> MVPISPIETVPVKLKPGMDGPKVKQWPLTEEKIKALVEICTEMEKEGKISKIGPENPYNTPVFACKKKDSTKWRKLVDFRELNKRTQDFWEVQLGIPHPAGLKKKKSVTVLDVGDAYFSVPLDEDFRKYTAFTIPSINNETPGIRYQYNVLPQGWKGSPAIFQSSMTKILEPFKKQNPDIVIYQYIDDLYVGSDLEIGQHRTKIEELRQHLLRWGLTTPDKKHQKEPPFLWMGYELHPDKWTVQPIVLPEKDSWTVNDIQKLVGKLNWASQIYPGIKVRQL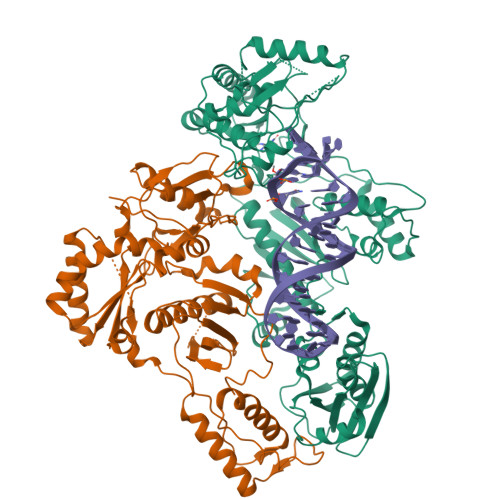SKLLRGTKALTEVIPLTEEAELELAENREILKEPVHGVYYDPSKDLIAEIQKQGQGQWTYQIYQEPFKNLKTGKYARMRGAHTNDVKQLTEAVQKITTESIVIWGKTPKFKLPIQKETWETWWTEYWQATWIPEWEFVNTPPLVKLWYQLEKEPIVGAETFYVDGAANRETKLGKAGYVTNKGRQKVVPLTNTTNQKTELQAIYLALQDSGLEVNIVTNSQYALGIIQAQPDKSESELVNQIIEQLIKKEKVYLAWVPAHKGIGGNEQVDKLVSA;> PISPIETVPVKLKPGMDGPKVKQWPLTEEKIKALVEICTEMEKEGKISKIGPENPYNTPVFAIKKKDSTKWRKLVDFRELNKRTQDFWEVQLGIPHPAGLKKKKSVTVLDVGDAYFSVPLDEDFRKYTAFTIPSINNKTPGIRYQYNVLPQGWKGSPAIFQSSMTKILEPFKKQNPDIVIYQYMDDLYVGSDLEIGQHRTKIEELRQHLLRWGLTTPDKKHQKEPPFLWMGYELHPDKWTVQPIVLPEKDSWTVNDIQKLVGKLNWASQIYPGIKVRQLSKLLRGTKALTEVIPLTEEAELELAENREILKEPVHGVYYDPSKDLIAEIQKQGQGQWTYQIYQEPFKNLKTGKYARMRGAHTNDVKQLTEAVQKITTESIVIWGKTPKFKLPIQKETWETWWTEYWQATWIPEWEFVNTPPLVKLWYQ> QKQYWVCNSSDASISYTYCDKMQYPISINVNPCIELKGSKGLLHIFYIPRRDLKQLYFNLYITVNTMNLPKRKEVICRGSDDDYSFCRALKGETVNTT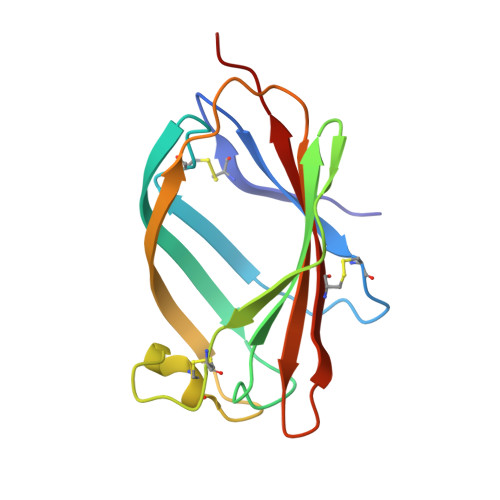ISFSFKGIKFSKGKYKCVVEAISGSPEEMLFCLEFVILHQPN> MDQKNGNMINLTTDKAVYQAGEAVHLNLTLNNTTSLAQNITATAEVYSLENKLKTLQYTKYLLPNESYTTQKGEFVIPANSLANNRGYLLKVNISDSQNNILEQGNRAIAVEDDWRTFPRYAAIGGSQKDNNSVLTKNLPDYYRELEQMKNMNINSYFFYDVYKSATNPFPNVPKFDQSWNWWSHSQVETDAVKALVNRVHQTGAVAMLYNMILAQNANETAVLPDTEYIYNYETGGYGQNGQVMTYSIDDKPLQYYYNPLSKSWQNYISNAMAQAMKNGGFDGWQGDTIGDNRVLSHNQKDSRDIAHSFMLSDVYAEFLNKMKEKLPQYYLTLNDV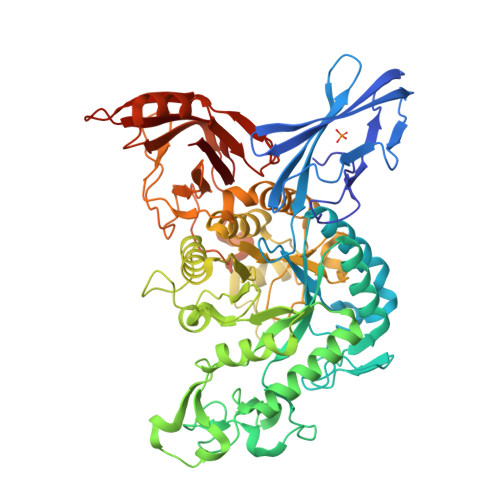NGENISKLANSKQDVIYNELWPFGTSALGNRPQESYGDLKARVDQVRQATGKSLIVGAYMEEPKFDDNRIPLNGAARDVLASATYQTDAVLLTTAAIAAAGGYHMSLAALANPNDGGGVGVLETAYYPTQSLKVSKELNRKNYHYQQFITAYENLLRDKVENDSAEPQTFTANGRQLSQDALGINGDQVWTYAKKGNDFRTIQLLNLMGITSDWKNEDGYENNKTPDEQTNLLVTYPLTGVSMAEADRIAKQVYLTSPDDWLQSSMISLATQVKTNENGDPVLYIQVPRLTLWDMIYILEHHHHHH> MKLLTTAILSSAIALSSMAAAAGTDNPTVAK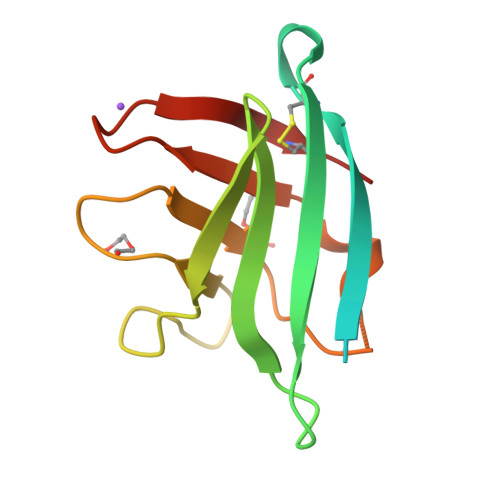KTVSYVCQQGKKVKVTYGFNKQGLTTYASAVINGKRVQMPVNLDKSDNVETFYGKEGGYVLGTGVMDGKSYRKQPIMITAPDNQIVFKDCSPR>[2x]MNLPTAQEVQGLMARYIELVDVGDIEAIVQMFADDATVEDPFGQPPIHGREQIAAFYRQGLGGGKVRAC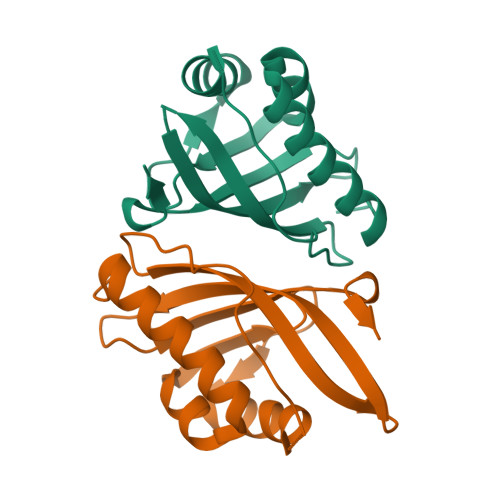LTGPVRASHNGCGAMPFRVEMVWNGQPCALDVILVMRFDEHGRIQTMQAYWSEVNLSVREPQ>[4x]GAASKKVNVLVVGLDNSGKTTIIERLKPRPRQAAEVAPTVGFTVDEVEKGPLTFTVFDMSGAGRYRTLWEQYYREADAVVFVVDSADKLRMVVARDEMEHMLKHSNMRKVPILYFANKKDLPVAMPPVEIAQALGLDDI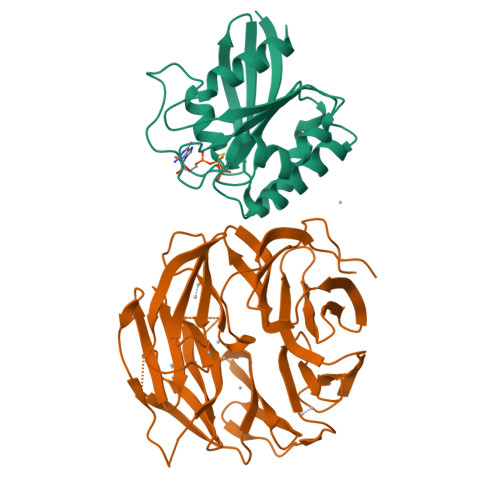KDRPWQIVPSNGLTGEGVDKGIDWLAERLS;>MVHESNPNDYAAGDAGNASGRYTTGSNGIPPMLPSVRSVWLDAFNDPVAGISAYTPCVHTCNLFGDGENRLVIADEDRKLKIWKGTQKASEHPLLDTPVAICSYISENTAPRLPALAVAAGSHIYIYRNLRPYYKFVLPPENVNTEEQDIWQKVMEGEIVIGEAVAQLTRLQVRAGDAGVVLQTRSLQLMNIGDPDAKMAFVEHWQGQPLVATTVITCMDVVKQAIDEPDAVSCLVVGTESGRILILNPAGTAIVKNIWVGITPAMIAVQGELDVGYRITVAGRDGKLYHIRNGELSQTIIQLEAQPVGLVRLAKHVAVGCMNDVVHAYTPTGHKSWSLYLPCHILAMQRMEVTGQRNTKALIVALSNGEVRVYNEKLLVSVHVSPNPVTALWFGRYGREDNTLLAITKSGALDIKMLPRTANLE[4x]>[6x]CEVDALKGTN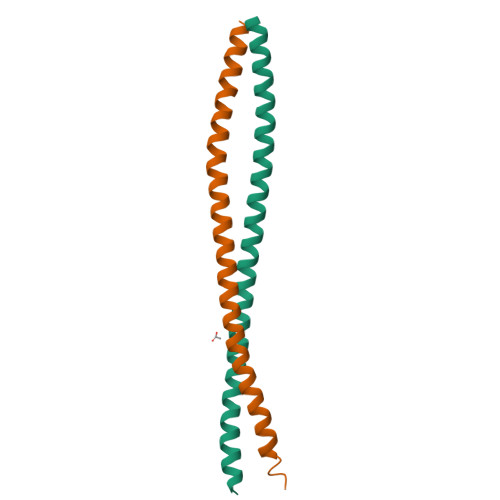ESLERQMREMEENFAVEAANYQDTIGRLQDEIQNMKEEMARHLREYQDLLNVKMALDIEIATYRKLLEGEESRI>[4x]PSVYDAAAQLTADVKKDLRDSWKVIGSDKKGNGVALMTTLFADNQETIGYFKRLGNVSQGMANDKLRGHSITLMYAL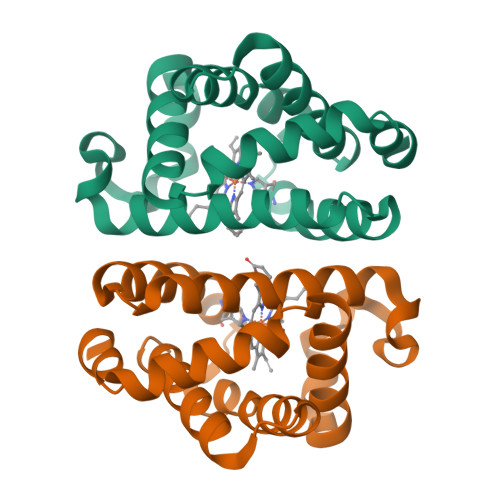QNFIDQLDNPDDLVCVVEKFAVNHITRKISAAEFGKFNGPIKKVLASKNFGDKYANAWAKLVAVVQAAL>[4x]MEELQDDYEDMMEENLEQEEYEDPDIPESQMEEPAAHDTEATATDYHTTSHPGTHKVYVELQELVMDEKNQELRWMEAARWVQLEENLGENGAWGRPHLSHLTFWSLLELRRVFTKGTVLLDLQETSLAGVANQLLDRFIFEDQIRPQDREELLRALLLKHSHAGELEALGGVKPAVLTRSGDPSQPLLPQHSSLETQLFCEQGDGGTEGHSPSGILEKIPPDSEATLVLVGRADFLEQPVLGFVRLQEAAELEAVELPVPIRFLFVLLGPEAPHIDYTQLGRAAATLMSERVFRIDAYMAQSRGELLHSLEGFLDCSLVLPPTDAPSEQALLSLVPVQRELLRRRYQSSPAKPDSSFYKGLDLNGGPDDPLQQTGQLFGGLVRDIRRRYPYYLSDITDAFSPQVLAAVIFIYFAALSPAITFGGLLGEKTRNQMGVSELLISTAVQGILFALLGAQPLLVVGFSGPLLVFEEAFFSFCETNGLEYIVGRVWIGFWLILLVVLVVAFEGSFLVRFISRYTQEIFSFLISLIFIYETFSKLIKIFQDHPLQKTYNYNVLMVPKPQGPLPNTALLSLVLMAGTFFFAMMLRKFKNSSYFPGKLRRVIGDFGVPISILIMVLVDFFIQDTYTQKLSVPDGFKVSNSSARGWVIHPLGLRSEFPIWMMFASALPALLVFILIFLESQITTLIVSKPERKMVKGSGFHLDLLLVVGMGGVAALFGMPWLSATTVRSVTHANALTVMGKASTPGAAAQIQEVKEQRISGLLVAVLVGLSILMEPILSRIPLAVLFGIFLYMGVTSLSGIQLFDRILLLFKPPKYHPDVPYVKRVKTWRMHLFTGIQIICLAVLWVVKSTPASLALPFVLILTVPLRRVLLPLIFRNVELQCLDADDAKATFDEEEGRDEYDEVAMPV;> MGQALGIKSCDFQAARNNEEHHTKALSSRRLFVRRGQPFTIILYFRAPVRAFLPALKKVALTAQTGEQPSKINRTQATFPISSLGDRKWWSAVVEERDAQSWTISVTTPADAVIGHYSLLLQVSGRKQLLLGQFTLLFNPWNREDAVFLKNEAQRMEYLLNQNGLIYLGTADCIQAESWDFGQFEGDVIDLSLRLLSKDKQVEKWSQPVHVARVLGALLHFLKEQRVLPTPQTQATQEGALLNKRRGSVPILRQWLTGRGRPVYDGQAWVLAAVACTVLRCLGIPARVVTTFASAQGTGGRLLIDEYYNEEGLQNGEGQRGRIWIFQTSTECWMTRPALPQGYDGWQILHPSAPNGGGVLGSCDLVPVRAVKEGTLGLTPAVSDLFAAINASCVVWKCCEDGTLELTDSNTKYVGNNISTKGVGSDRCEDITQNYKYPEGSLQEKEVLERVEKEKMEREKDNGIRPPSLETASPLYLLLKAPSSLPLRGDAQISVTLVNHSEQEKAVQLAIGVQAVHYNGVLAAKLWRKKLHLTLSANLEKIITIGLF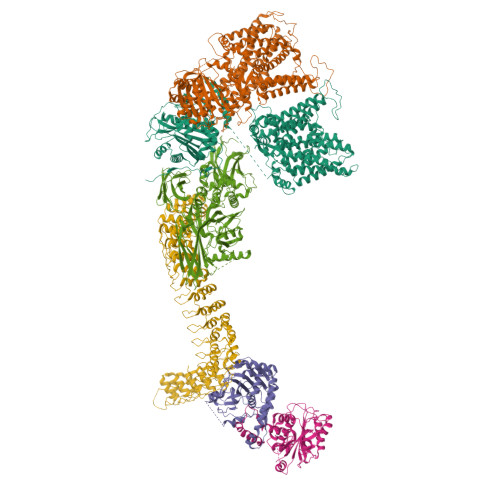FSNFERNPPENTFLRLTAMATHSESNLSCFAQEDIAICRPHLAIKMPEKAEQYQPLTASVSLQNSLDAPMEDCVISILGRGLIHRERSYRFRSVWPENTMCAKFQFTPTHVGLQRLTVEVDCNMFQNLTNYKSVTVVAPELSA;> MPYSVGFREADAATSFLRAARSGNLDKALDHLRNGVDINTCNQNGLNGLHLASKEGHVKMVVELLHKEIILETTTKKGNTALHIAALAGQDEVVRELVNYGANVNAQSQKGFTPLYMAAQENHLEVVKFLLENGANQNVATEDGFTPLAVALQQGHENVVAHLINYGTKGKVRLPALHIAARNDDTRTAAVLLQNDPNPDVLSKTGFTPLHIAAHYENLNVAQLLLNRGASVNFTPQNGITPLHIASRRGNVIMVRLLLDRGAQIETKTKDELTPLHCAARNGHVRISEILLDHGAPIQAKTKNGLSPIHMAAQGDHLDCVRLLLQYDAEIDDITLDHLTPLHVAAHCGHHRVAKVLLDKGAKPNSRALNGFTPLHIACKKNHVRVMELLLKTGASIDAVTESGLTPLHVASFMGHLPIVKNLLQRGASPNVSNVKVETPLHMAARAGHTEVAKYLLQNKAKVNAKAKDDQTPLHCAARIGHTNMVKLLLENNANPNLATTAGHTPLHIAAREGHVETVLALLEKEASQACMTKKGFTPLHVAAKYGKVRVAELLLERDAHPNAAGKNGLTPLHVAVHHNNLDIVKLLLPRGGSPHSPAWNGYTPLHIAAKQNQVEVARSLLQYGGSANAESVQGVTPLHLAAQEGHAEMVALLLSKQANGNLGNKSGLTPLHLVAQEGHVPVADVLIKHGVMVDATTRMGYTPLHVASHYGNIKLVKFLLQHQADVNAKTKLGYSPLHQAAQQGHTDIVTLLLKNGASPNEVSSDGTTPLAIAKRLGYISVTDVLKVVTDETSFVLVSDKHRMSFPETVDEILDVSEDEGEELISFKAERRDSRDVDEEKELLDFVPKLDQVVESPAIPRIPCAMPETVVIRSEEQEQASKEYDEDSLIPSSPATETSDNISPVASPVHTGFLVSFMVDARGGSMRGSRHNGLRVVIPPRTCAAPTRITCRLVKPQKLSTPPPLAEEEGLASRIIALGPTGAQFLSPVIVEIPHFASHGRGDRELVVLRSENGSVWKEHRSRYGESYLDQILNGMDEELGSLEELEKKRVCRIITTDFPLYFVIMSRLCQDYDTIGPEGGSLKSKLVPLVQATFPENAVTKRVKLALQAQPVPDELVTKLLGNQATFSPIVTVEPRRRKFHRPIGLRIPLPPSWTDNPRDSGEGDTTSLRLLCSVIGGTDQAQWEDITGTTKLVYANECANFTTNVSARFWLSDCPRTAEAVNFATLLYKELTAVPYMAKFVIFAKMNDPREGRLRCYCMTDDKVDKTLEQHENFVEVARSRDIEVLEGMSLFAELSGNLVPVKKAAQQRSFHFQSFRENRLAMPVKVRDSSREPGGSLSFLRKAMKYEDTQHILCHLNITMPPCAKGSGAEDRRRTPTPLALRYSILSESTPGSLSGTEQAEMKMAVISEHLGLSWAELARELQFSVEDINRIRVENPNSLLEQSVALLNLWVIREGQNANMENLYTALQSIDRGEIVNMLEGSGRQSRNLKPDRRHTDRDYSLSPSQMNGYSSLQDELLSPASLGCALSSPLRADQYWNEVAVLDAIPLAATEHDTMLEMSDMQVWSAGLTPSLVTAEDSSLECSKAEDSDATGHEWKLEGALSEEPRGPELGSLELVEDDTVDSDATNGLIDLLEQEEGQRSEEKLPGSKRQDDATGAGQDSENEVSLVSGHQRGQARITHSPTVSQVTERSQDRLQDWDADGSIVSYLQDAAQGSWQEEVTQGPHSFQGTSTMTEGLEPGGSQEYEKVLVSVSEHTWTEQPEAESSQADRDRRQQGQEEQVQEAKNTFTQVVQGNEFQNIPGEQVTEEQFTDEQGNIVTKKIIRKVVRQIDLSSADAAQEHEEVTVEGPLEDPSELEVDIDYFMKHSKDHTSTPNP>SMDDDQVAFSFILDNIVTQKMMAVPDSWPFHHPVNKKFVPDYYKVIVNPMDLETIRKNISKHKYQSRESFLDDVNLILANSVKYNGPESQYTKTAQEIVNVCYQTLTEYDEHLTQLEKDICTAKEAALEEAE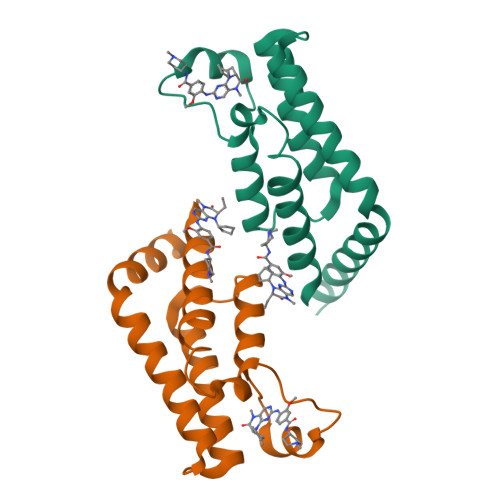LESLD[2x]> HGSMETPPSRVYGCFLEGPENPKSAACKAAVAAGGTQALYDWNGVNQGNANGNHQAVVPDGQLCGAGKALFKGLNLARSDWPSTAIAPDASGNFQFVYKASAPHATRYFDFYITKDGYNPEKPLAWSDLEPAPFCSITSVKLENGTYRMNCPLPQGKTGKHVIYNVWQRSDSPEAFYACIDVSFSG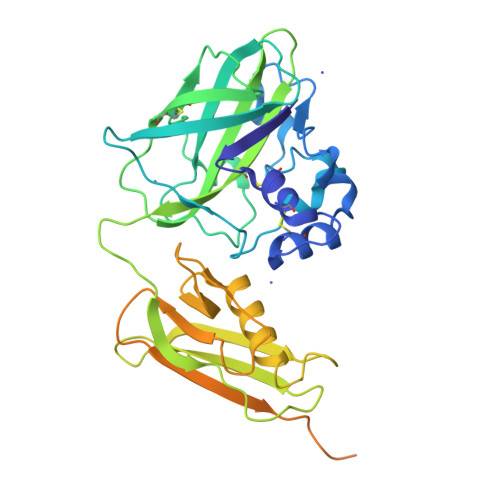AVANPWQALGNLRAQQDLPAGATVTLRLFDAQGRDAQRHSLTLAQGANGAKQWPLALAQKVNQDSTLVNIGVLDAYGAVSPVASSQDNQVYVRQAGYRFQVDIELPVEGGGEQPGGDGKVDFDYPQGLQQYDAGTVVRGADGKRYQCKPYPNSGWCKGWDLYYAPGKGMAWQDAWTLLHHHHHHHHHH> SGRPMTLQSAMGDMYQSIFVATPPLLQMEQEQPFPELIRTWAGLLGQIGVESVRTEEVNFGQLAKCFNDYLNTVAEHCEQQNIWQHKREENHNFFTAFKPDASKAALHGHAYIAHYKESVILRHLSIVDPKTLGMLRFAPYEAPSTDYCRHFPDSPWAKMQRLA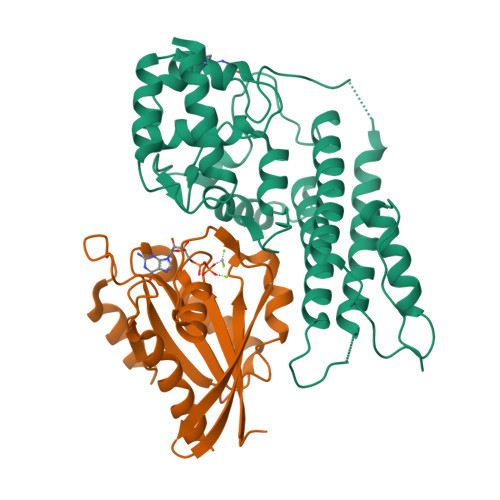TAGQNIILQLRLIQNGQMLEDDFMKEKLPVLQKALDDFMQYKTEVDALLAHDSEVTPVSTHDSSFFYDIDEQTLNAMSGDQLATICFEELNAPHPSRLIMRILKSDSLWQEVDDSLNGDAFMGRQDDICEKRNKICQWRQLVQMTT;> SGRPMSSMNPEYDYLFKLLLIGDSGVGKSCLLLRFADDTYTESYISTIGVDFKIRTIELDGKTIKLQIWDTAGQERFRTITSSYYRGAHGIIVVYDVTDQESFNNVKQWLQEIDRYASENVNKLLVGNKCDLTTKKVVDYTTAKEFADSLGIPFLETSAKNATNVEQSFMTMAAEIKKRMG> RIKKISIEGNIAAGKSTFVNILKQLCEDWEVVPEPVARWCNVQSTQ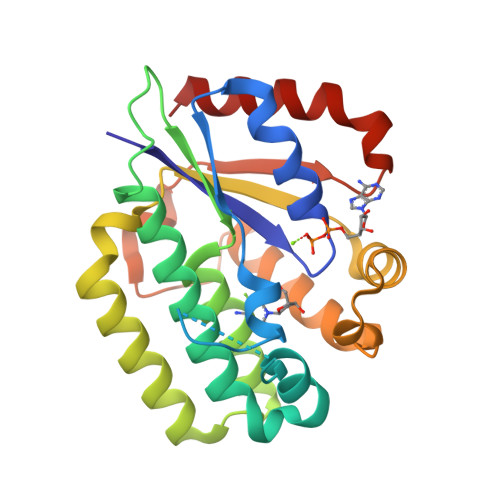DEFEELTMSQKNGGNVLQMMYEKPERWSFTFQTYACLSRIRAQLASLNGKLKDAEKPVLFFERSVYSDRYIFASNLYESECMNETEWTIYQDWHDWMNNQFGQSLELDGIIYLQATPETCLHRIYLRGRNEEQGIPLEYLEKLHYKHESWLLHRTLKTNFDYLQEVPILTLDVNEDFKDKYESLVEKVKEFLSTL> MASMERFLSVYDEVQAFLLDQLQSKYEIDPNRARYLRIMMDTTCLGGKYFRGMTVVNVAEGFLAVTQHDEATKERILHDACVGGWMIEFLQAHYLVEDDIMDGSVMRRGKPCWYRFPGVTTQCAINDGIILKSWTQIMAWHYFADRPFLKDLLCLFQKVDYATAVGQMYDVTSMCDSNKLDPEVAQPMTTDFAEFTPAIYKRIVKYKTTFYTYLLPLVMGLLVSEAAASVEMNLVERVAHLIGEYFQVQDDVMDCFTPPEQLGKVGTDIEDAK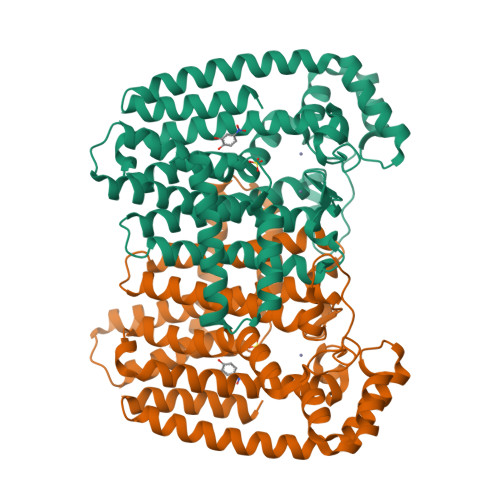CSWLAVTFLGKANAAQVAEFKANYGEKDPAKVAVVKRLYSKANLQADFAAYEAEVVREVESLIEQLKVKSPTFAESVAVVWEKTHKRKK Pendrin (SLC26A4) is an anion exchanger expressed in the apical membranes of selected epithelia. Encoded by the gene SLC26A4, pendrin belongs to the solute carrier 26 (SLC26) family. Pendrin ablation causes Pendred syndrome, a genetic disorder associated with sensorineural hearing loss, hypothyroid goiter, and reduced blood pressure.

Similarly, the pendrin sample in the anion pair of Cl−/I− (1:3) (pendrin-Cl/I) was prepared and used for structure determination. Symmetric inward-open and asymmetric homodimers were observed with approximate percentage of 75 and 25%, respectively. After superimposing all structures we resolved, we found very little difference among inward-open structures or among outward-open structures, respectively, with root mean squared deviation (RMSD) no more than 0.5 Å. The symmetric inward-open conformation most likely represents the energetically favorite state, existing in the single binding-anion condition, Cl− for instance.

>MAARGGRSEPPQLAEYSCSYTVSRPVYSELAFQQQRERRLPERRTLRDSLARSCSCSRKRAFGVVKTLLPILDWLPKYRVKEWLLSDIISGVSTGLVGTLQGMAYALLAAVPVQFGLYSAFFPILTYFVFGTSRHISVGPFPVVSLMVGSVVLSMAPDDHFLVPSGNGSALNSTTLDTGTRDAARVLLASTLTLLVGIIQLVFGGLQIGFIVRYLADPLVGGFTTAAAFQVLVSQLKIVLNVSTKNYNGILSIIYTLIEIFQNIGDTNIADFIAGLLTIIVCMAVKELNDRFKHRIPVPIPIEVIVTIIATAISYGANLEKNYNAGIVKSIPSGFLPPVLPSVGLFSDMLAASFSIAVVAYAIAVSVGKVYATKHDYVIDGNQEFIAFGISNVFSGFFSCFVATTALSRTAVQESTGGKTQVAGLISAVIVMVAIVALGRLLEPLQKSVLAAVVIANLKGMFMQVCDVPRLWKQNKTDAVIWVFTCIMSIILGLDLGLLAGLLFALLTVVLRVQFPSWNGLGSVPSTDIYKSITHYKNLEEPEGVKILRFSSPIFYGNVDGFKKCINSTVGFDAIRVYNKRLKALRRIQKLIKKGQLRATKNGIISDIGSSNNAFEPDEDVEEPEELNIPTKEIEIQVDWNSELPVKVNVPKVPIHSLVLDCGAVSFLDVVGVRSLRMIVKEFQRIDVNVYFALLQDDVLEKMEQCGFFDDNIRKDRFFLTVHDAILHLQNQVKSREGQDSLLETVARIRDCKDPLDLMEAEMNAEELDVQDEAMRRLAS[2x]~{N}-(1-ethylbenzimidazol-2-yl)ethanamide | C11 H13 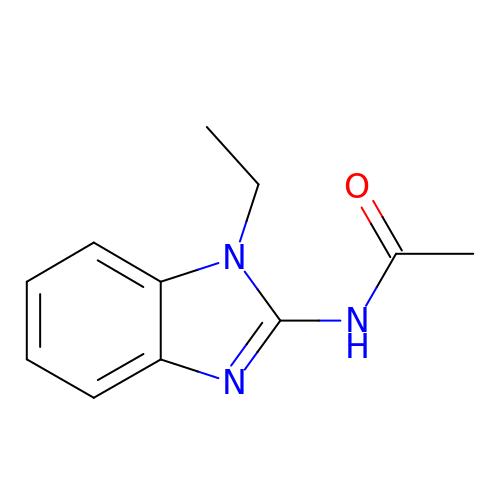N3 O | CTAOPYAHPUKQBH-UHFFFAOYSA-N The periplasmic binding protein (PBP) CeuE1 is an important component of the Fe(III) uptake system in Campylobacter jejuni, a commensal Gram-negative bacterium in the avian gut, but a common source of food poisoning in humans. CeuE, an integral part of the CeuBCDE ABC transporter of C. jejuni, is responsible for capturing Fe(III)-siderophore complexes in the periplasm for delivery to their respective inner membrane transporter. C. jejuni does not itself synthesize siderophores, but capitalizes on their secretion by other bacteria, such as E. coli. Here we report a combined solution and structural study of a series of synthetic tetradentate analogues of the enterobactin-derived bis(2, 3-dihydroxybenzoyl-L-Ser), to explore the ligand-binding promiscuity of CeuE, both wild type and with mutations of the Fe(III) binding residues H227 and Y288.

To probe the relative contributions of His227 and Tyr288 to Fe(III)-siderophore binding, site-directed mutagenesis was then used to replace the side chains of the two Fe(III)-coordinating amino acids with non-coordinating side chains of similar size. His227 was mutated to either leucine (H227L) or alanine (H227A), while Y288 was mutated to phenylalanine (Y288F). All five mutants (Y288F, H227L, H227A, H227L/Y288F, H227A/Y288F) were crystallized in their apo form, and all structures are closely similar to that of wild type CeuE. However while there is clear electron density for the Y288F mutation in its three structures, H227L and H227A are located in a flexible loop region and there is generally no electron density to confirm their presence. In contrast, the effect of mutating the histidine was less pronounced. Mutants H227L and H227A gave Kd values of 22 ± 10 nM and 35 ± 14 nM, respectively, indicating only slightly weaker binding than for wild type, which indicates that the tyrosinate O-donor binds the Fe(III) cation more strongly than the histidine N-donor. The Λ-configuration signal was observed for mutants H227L and H227A, indicating that these do indeed bind Λ-Fe-5-Lic. The resulting Kd values show trends similar to that observed for wild type, but with systematically weaker binding.

>GPAMLPISMSDEGDSFLVKDSLGENKIPKNPSKVVILDLGILDTFDALKLNDKVVGVPAKNLPKYLQQFKNKPSVGGVQQVDFEAINALKPDLIIISGRQSKFYDKLKEIAPTLFVGLDNANFLSSFENNVLSVAKLYGLEKEALEKISDIKNEIEKAKSIVDEDKKALIILTNSNKISAFGPQSRFGIIHDVLGINAVDENIKVGTAGKSINSEFILEKNPDYIFVVDRNVILGNKERAQGILDNALVAKTKAAQNKKIIYLDPEYWYLASGNGLESLKTMILEIKNAVK[3x]>MQQGQMAYDRAITVFSPDGRLFQVEYAREAVKKGSTALGMKFANGVLLISDKKVRSRLIEQNSIEKIQLIDDYVAAVTSGYVADARVLVDFARISAQQEKVTYGSLVNIENLVKRVADQMQQYTQYGGVRPYGVSLIFAGIDQIGPRLFDCDPAGTINEYKATAIGSGKDAVVSFLEREYKENLPEKEAVTLGIKALKSSLEEGEELKAPEIASITVGNKYRIYDQEEVKKFL[14x];>MNQTLETGTTTVGITLKDAVIMATERRVTMENFIMHKNGKKLFQIDTYTGMTIAGLVGDAQVLVRYMKAELELYRLQRRVNMPIEAVATLLSNMLNQVKYMPYMVQLLVGGIDTAPHVFSIDAAGGSVEDIYASTGSGSPFVYGVLESQYSEKMTVDEGVDLVIRAISAAKQRDSASGGMIDVAVITRKDGYVQLPTDQIESRIRKLGLIL[14x]

The ubiquitin-proteasome system (UPS) is a crucial regulatory pathway responsible for eliminating damaged or unnecessary proteins within cells. Central to this system is the proteasome, a molecular machine that selectively degrades proteins. A hydrophobic-tyrosine-any residue (HbYX) motif on the C-termini of proteasome-activating complexes independently triggers gate-opening of the 20S core particle for protein degradation; however, the causal allosteric mechanism remains unclear. The architecture of the archaeal 20S proteasome is conserved resembling the eukaryotic 20S, but its α and β rings are homoheptameric rather than heteroheptameric.

Understanding the critical role of tyrosine in the HbYX motif, and recognizing the partial activation caused by the L81Y mutation—which was designed to mimic the tyrosine occupancy of HbYX, as identified in a concurrent study31—we moved forward with constructing a cryo-EM structure of T20S-αL81Y. Unlike the ZYA-T20S model, the conformational changes caused by L81Y were different and subtle. We did not observe a substantial α-ring rotation or a conformational change at the loop proximal to K66; however, we did observe a slight rise of Helix 0 in a direction parallel with the sevenfold axis mostly clearly seen in Fig. 5b. The T20S-αL81Y model shows that the hydroxyl group of tyrosine is within proximity to hydrogen bond with the backbone of G19, similar to ZYA’s tyrosine. Additionally, we noted that tyrosine hydrogen bonded with a water molecule that is also hydrogen bonding to the backbone of L21 but not the side chain of E25. We also noted the water which hydrogen bonds with the backbone of A30 is not displaced by L81Y, reinforcing the point that L81Y is not oriented like ZYA’s tyrosine. This structure suggests that the tyrosine interactions with G19 and L21 are sufficient to cause a Helix 0 shift upward, which consequently partially opens the gate. Therefore, the L81Y tyrosine by itself cannot fully mimic the ZYA-bound open state.>[2x]MELIQDTSRPPLEYVKGVPLIKYFAEALGPLQSFQARPDDLLISTYPKSGTTWVSQILDMIYQGGDLEKCHRAPIFMRVPFLEFKAPGIPSGMETLKDTPAPRLLKTHLPLALLPQTLLDQKVKVVYVARNAKDVAVSYYHFYHMAKVHPEPGTWDSFLEKFMVGEVSYGSWYQHVQEWWELSRTHPVLYLFYEDMKENPKREIQKILEFVGHSLPEETVDFMVQH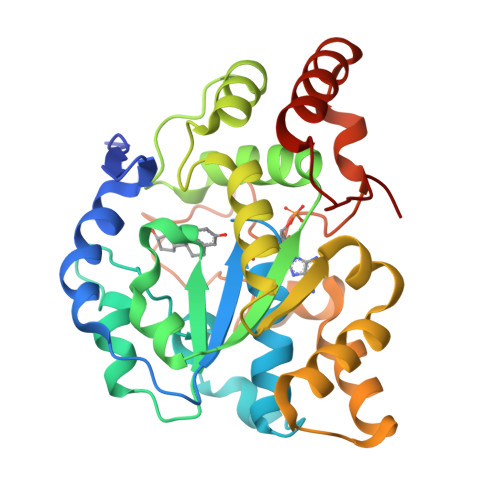TSFKEMKKNPMTNYTTVPQEFMDHSISPFMRKGMAGDWKTTFTVAQNERFDADYAEKMAGCSLSFRSEL>[2x]MDTPNKDDSIIRFSVSLQQNLLDELDNRIIKNGYSSRSELVRDMIREKLVEDNWAEDNPNDESKIAVLVVIY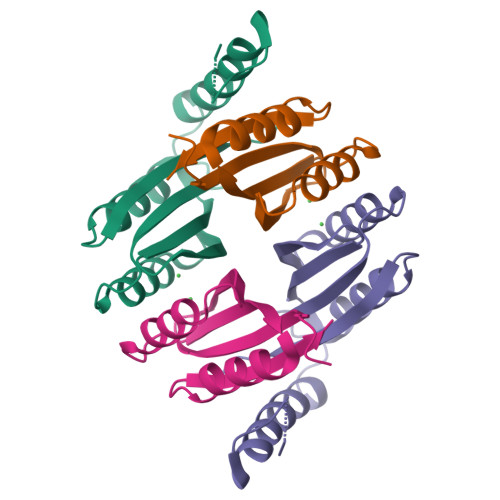DAHQRELNQRMIDIQHASGTHVLCTTHIHMDEHNCLETIILQGNSFEIQRLQLEIGGLRGVKFAKLTKASSFEYNE> MKIYIQPLSVNSHTVEVLANSLPKIFNAEVFVLPASDVSLKCYNASRRQYNSTCILRMLPPIKVTLGVTGKDIYAKGMNFVFGEAELGGARAVLSVFRLTTADSELYRERVVKEAVHEIGHVLGLKHCSNNCVMRFSNSVQDVDRKPVSFCRECASKIRY

Archaemetzincins are metalloproteases occurring in archaea and some mammalia. They are distinct from all the other metzincins by their extended active site consensus sequence HEXXHXXGXXHCX4CXMX17CXXC featuring four conserved cysteine residues. The overall structure of AfAmzA resembles those of other metzincins, consisting of an upper N-terminal domain (NTD) and a lower helical C-terminal domain (CTD) with respect to the active site helix α2, which harbors two of the three zinc-binding histidines (H117EIGH121) and the catalytic base Glu118. On the other hand, as the homologous archaemetzincins from Methanopyrus kandleri (MkAmzA) and Methanocorpusculum labreanum (MlAmzA), AfAmzA exhibits a second zinc-binding site located in the CTD immediately below the catalytic zinc binding site and close to the eponymous, structurally important Met-turn.

Consequently, two different crystal forms are observed, one triclinic and one hexagonal. In the nat-AfAmzA::citrate complex the catalytic zinc ion is penta-coordinated in a either slightly distorted square pyramidal or a bidentate tetrahedral geometry by three histidine imidazoles as well as by the carbonyl oxygen (Oβ1) and hydroxyl oxygen (OHβ) of citrate, with ligand-metal distances of 2.0–2.2 Å. The catalytic water molecule is completely excluded from the zinc environment. In the case of citrate as zinc ligand, the S1′-wall forming segment has to move to avoid steric clashes with the pro-S -CH2-COO- branch of the ligand. This has also been observed in a citrate-bound crystal form of the related M. kandleri archaemetzincin. Besides acting as zinc ligands, these carboxylic acids also mediate a new crystal contact consisting of a salt bridge between one of their carboxylate groups and Arg152 of a symmetry-related molecule. As a consequence, significant differences are observed between NHis-AfAmzA and the two carboxylate-coordinated nat-AfAmzA crystal forms. On the other hand, we detect upon ligand binding opening of the active site at the S' sites.> MLQFEIDDEMEPLYNQAKQMRYGDYMKSTFKEDHSLEHRCVESAKIRAKY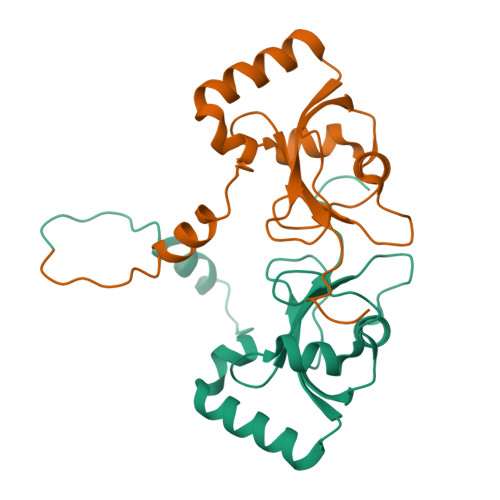PDRVPVIVEKVSGSQIVDIDKRKYLVPSDITVAQFMWIIRKRIQLPSEKAIFLFVDKTVPQSSLTMGQLYEKEKDEDGFLYVAYSGENTFGLEVLFQ(3R)-4-(3,5-dimethylphenyl)-N-(2-methoxyphenyl)-3-methylbutanamide 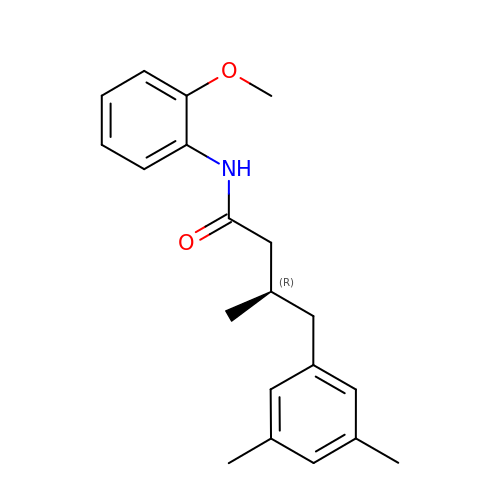| C20 H25 N O2 | XJYBAKSVSQKCNC-MRXNPFEDSA-N> GVMTDVHRRFLQLLMTHGVLEEWDVKRLQTHCYKVHDRNATVDKLEDFINNINSVLESLYIEIKRGVTEDDGRPIYALVNLATTSISKMATDFAENELDLFRKALELIIDSETGFASSTNILNLVDQLKGKKMRKKEAEQVLQKFVQNKWLIEKEGEFTLHGRAILEMEQYIRETYPDAVKICNICHSLLIQGQ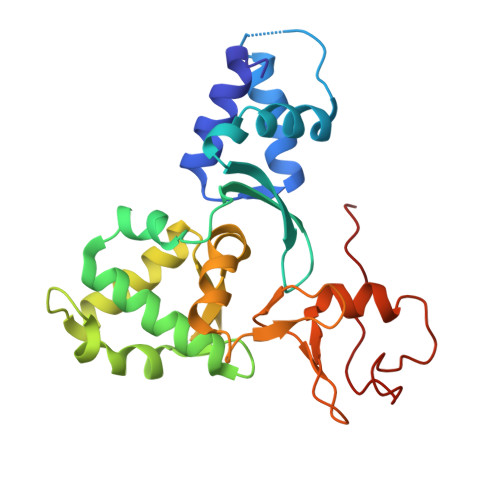SCETCGIRMHLPCVAKYFQSNAEPRCPHCNDYWPHEIPKVFDPE> AAAALAQPVEWTPCRSSNPQVKIPGGALCGKLAVPVDYDRPDGDVAALALIRFPATGDKIGSLVINPGGPGESGIEAALGVFQTLPKRVHERFDLVGFDPRGVASSRPAIWCNSDADNDRLRAEPQVDYSREGVAHIENETKQFVGRCVDKMGKNFLAHVGTVNVAKDLDAIRAALGDDKLTYLGYSYGTRIGSAYAEEFPQRVRAMILDGAVDPNADPIEAELRQAKGFQDAFNNYAADCAKNAGCPLGADPAKAVEVYHSLVDPLVDPDNPRISRPARTKDPRGLSYSDAIVGTIMALYSPNLWQHLTDGLSELVDNRGDTLLALADMYMRRDSHGRYNNSGDARVAINCVDQPPVTDRDKVIDEDRRAREIAPFMSYGKFTGDAPLGTCAFWPVPPTSQPHAVSAPGLVPTVVVSTTHDPATPYKAGVDLANQLRGSLLTFDGTQHTVVFQGDSCIDEYVTAYLIG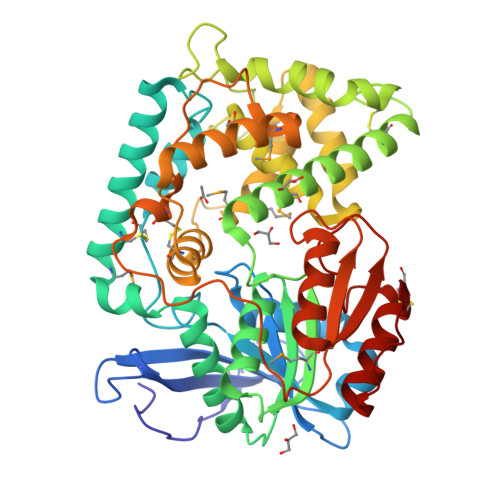GTTPPSGAKC> GSAMGSSDEPRDDFKEAVNAFNPNPIEKWTGRFNTENASVRRRTLNVPGFKSIPTVYTEATLPLNKDVTDGRLTVVVNINTVQPFTRRTPLRVKREKWYTCSSSQCSGSSSKCDCHRKHDEFRNKCISEGGRYTTESSKCRLGEKCGYCKQNVYLATLYLVAGSVGGGMYRESDKYQSALYPFYDISQGYEPRQPSSVNVRLYSEGDPFIAFQQLTEGREEFG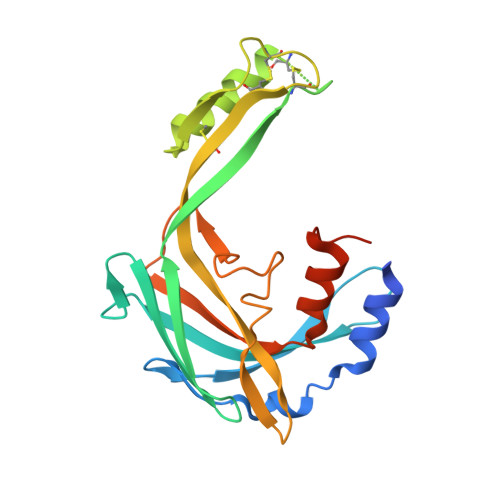IPNRTVGAAA> MSTGDFLTKGIELVQKAIDLDTATQYEEAYTAYYNGLDYLMLALKYEKNPKSKDLIRAKFTEYLNRAEQLKKHLESEEANAAKKSPSAGSGSNGGNKKISQEEGEDNGGEDNKKLRGALSSAILSEKPNVKWEDVAGLEGAKEALKEAVILPVKFPHLFKGNRKPTSGILLYGPPGTGKSYLAKAVATEANSTFFSVSSSDLVSKWMGESEKLVKQLFAMARENKPSIIFIDEVDALTGTRGEGESEASRRIKTELLVQMNGV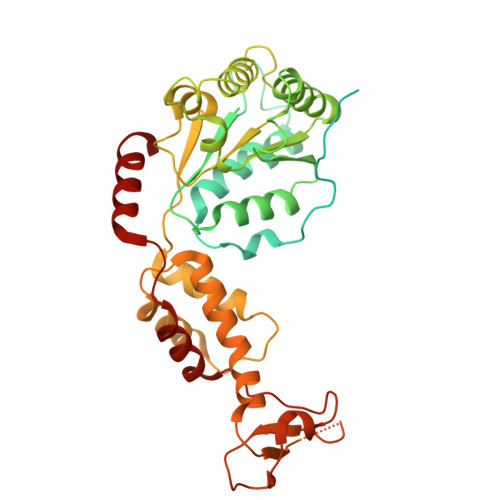GNDSQGVLVLGATNIPWQLDSAIRRRFERRIYIPLPDLAARTTMFEINVGDTPCVLTKEDYRTLGAMTEGYSGSDIAVVVKDALMQPIRKIQSATHFKDVSTEDDETRKLTPCSPGDDGAIEMSWTDIEADELKEPDLTIKDFLKAIKSTRPTVNEDDLLKQEQFTRDFGQEGN>[2x]MTPIETVTAFIAHWNSGDMEAMYDLCAEDVVWHNIPMEPIAGKPAMRAAVEGFMANVSQCDWQVHAIAANGATVLTERTDGFTFTNGRRATIRVMGTFEC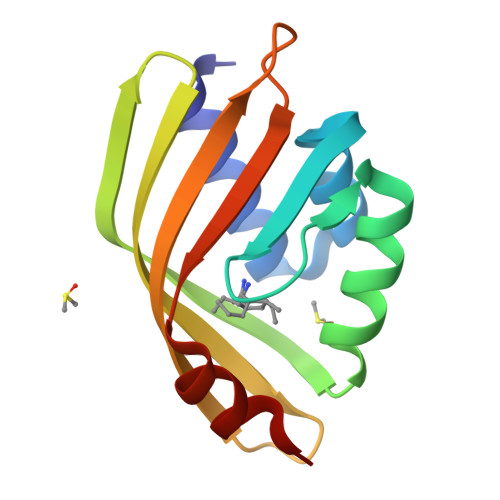DAERRIIAWRDYFDMLEFQREFAGA>[2x]SGDRSMVEVLADHPGELVRTDSPNFLSSVLPTHWRSNKTLPIAFKVVALGDVPDGTLVTVMAGNDENYSAELRNATAAM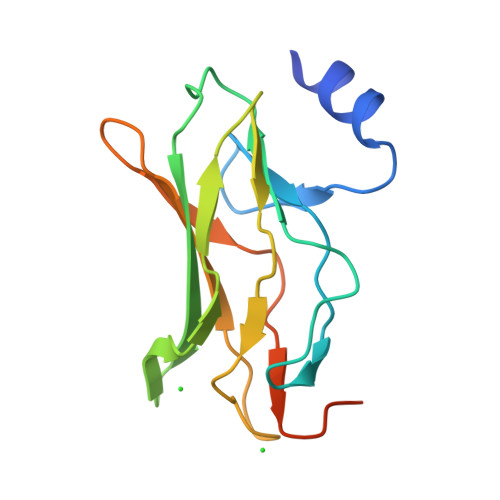KNQVARFNDLRFVGRSGRGKSFTLTITVFTNPPQVATYHNAIKITVDGPREPRRHRQKLDD2-[4-(2,5-Dioxopyrrolidin-1-yl)phenoxy]acetate 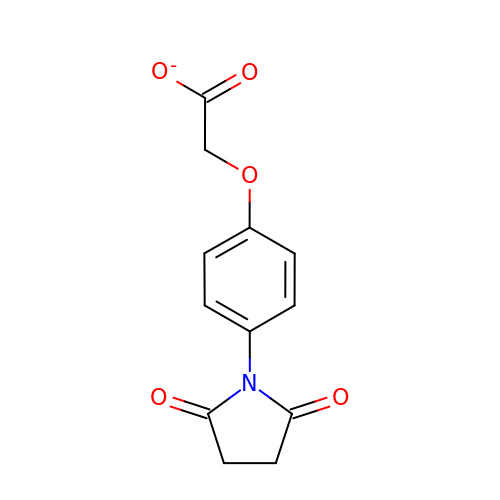| C12 H10 N O5 | DVXARNQLROBEQU-UHFFFAOYSA-M> GSDELYRQSLEIISRYLREQATGAKDTKPMGRSGATSRKALETLRRVGDGVQRNHETAFQGMLRKLDIKNEDDVKSLSRVMIHVFSDGVTNWGRIVTLISFGAFVAKHLKTINQESCIEPLAESITDVLVRTKRDWLVKQRGWDGF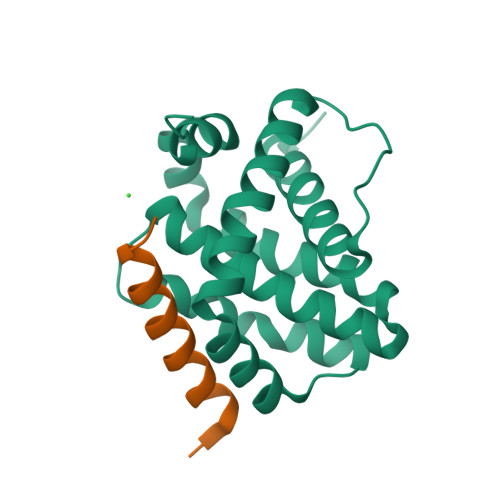VEFFHVED;> XDKTLEEIARELLKLALEIDKEIX> STQVCTGTDMKLRLPASPETHLDMLRHLYQGCQVVQGNLELTYLPTNASLSFLQDIQEVQGYVLIAHNQVRQVPLQRLRIVRGTQLFEDNYALAVLDNGDPLNNTTPVTGASPGGLRELQLRSLTEILKGGVLIQRNPQLCYQDTILWKDIFHKNNQLALTLIDTNRSRACHPCSPMCKGSRCWGESSEDCQSLTRTVCAGGCARCKGPLPTDCCHEQCAAGCTGPKHSDCLACLHFNHSGICELHCPALVTYNTDTFESMPNPEGRYTFGASCVTACPYNYLSTDVGSCTLVCPLHNQEVTAEDGTQKCEKCSKPCARVCYGLGMEHLREVRAVTSANIQEFAGCKKIFGSLAFLP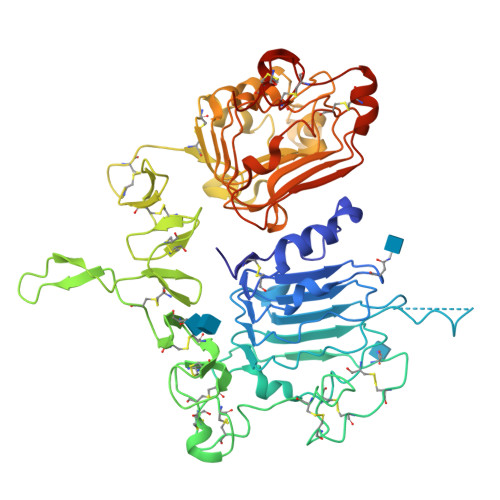ESFDGDPASNTAPLQPEQLQVFETLEEITGYLYISAWPDSLPDLSVFQNLQVIRGRILHNGAYSLTLQGLGISWLGLRSLRELGSGLALIHHNTHLCFVHTVPWDQLFRNPHQALLHTANRPEDECVGEGLACHQLCAKGHCWGPGPTQCVNDYKDDDDK>[4x]GPGSTGASLGMMWKDKLNAMTKEEFTRYKRAGVMETDRKEARDYLKRGDGKTGLSVSRGTAKLAWMEERGYVELTGRVVDLGCGRGGWSYYAASRPHVMDVRAYTLGVGGHEVPRITESYGWNIVKFKSRVDIHTLPVERTDVIMCDVGESSPKWSVESERTIKILELLEKWKVKNPSADFVVKVLCPYSVE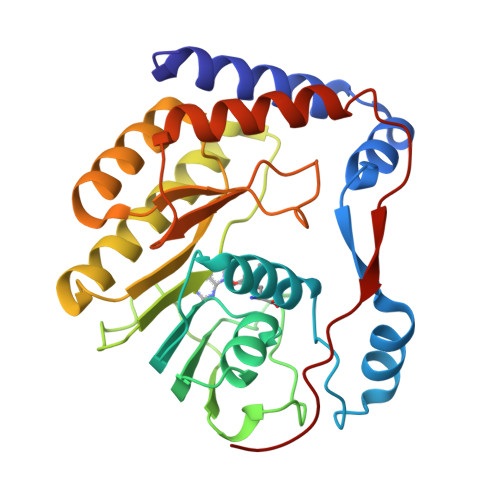VMERLSVMQRKWGGGLVRNPYSRNSTHEMYFTSRAGGNIIGAVTACTERLLGRMARRDGPVVVPELNLGTGTR> MGHHHHHHGSGSNRLDGKVAIITGGTLGIGLAIATKFVEEGAKVMITGRHSDVGEKAAKSVGTPDQIQFFQHDSSDEDGWTKLFDATEKAFGPVSTLVNNAGIAVNKSVEETETAEWRKLLAVNLDGVFFGTRLGIKRMKNKGLGASIINMSSIEGFVGDPSLGAYN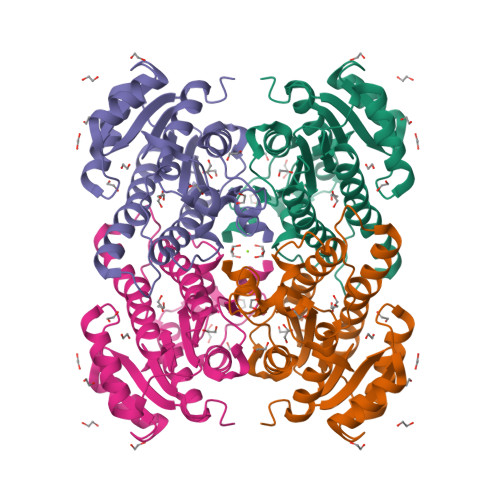ASKGAVRIMSKSAALDCALKDYDVRVNTVHPGYIKTPLVDDLPGAEEAMSQRTKTPMGHIGEPNDIAYICVYLASNESKFATGSEFVVDGGYTAQ> XXXXXXXXXXXXXXARELEELNVPGEIVESLSSSEESITRINKKIEKFQSEEQQQTEDELQDKIHPFAQTQSLVYPFPGPIPNSLPQNIPPLTQTPVVVPPFLQPEVMGVSKVKGAMAPKHKEMPFPKY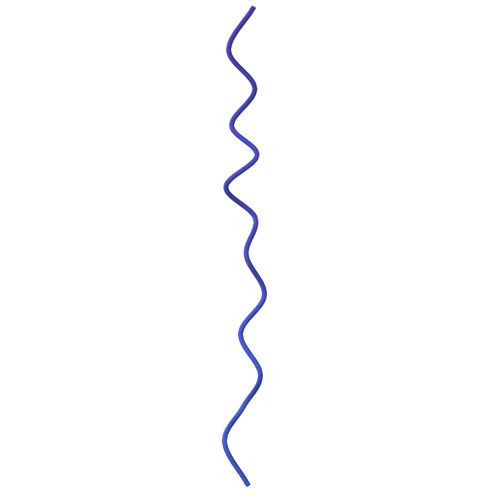PVEPLTESQSLTLTDVENLHLPLPLLQSWMHQPHQPLPPTVMFPPQSVLSLSQSKVLPVPQKAVPYPQRDMPIQAFLLYQEPVLGPVRGPFPIIV> MGSSHHHHHHSSGLVPRGSMATAPYNYSYIFKYIIIGDMGVGKSCLLHQFTEKKFMADCPHTIGVEFGTRIIEVSGQKIKLQIWDTAGQGRFRAVT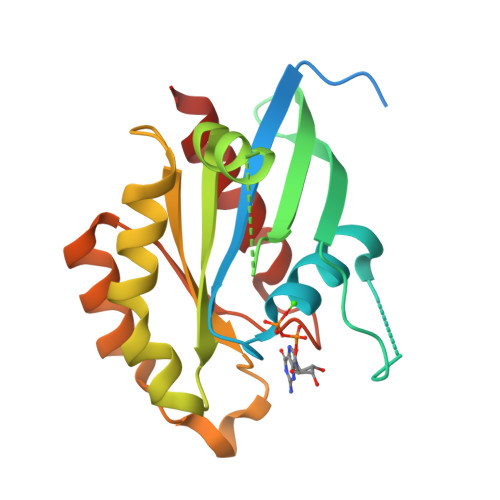RSYYRGAAGALMVYDITRRSTYNHLSSWLTDARNLTNPNTVIILIGNKADLEAQRDVTYEEAKQFAEENGLLFLEASAKTGENVEDAFLEAAKKIYQNIQ>[2x]MTSRDGYQWTPETGLTQGVPSLGVISPPTNIEDTDKDGPWDVIVIGGGYCGLTATRDLTVAGFKTLLLEARDRIGGRSWSSNIDGYPYEMGGTWVHWHQSHVWREITRYKMHNALSPSFNFSRGVNHFQLRTNPTTSTYMTHEAEDELLRSALHKFTNVDGTNGRTVLPFPHDMFYVPEFRKYDEMSYSERIDQIRDELSLNERSSLEAFILLCSGGTLENSSFGEFLH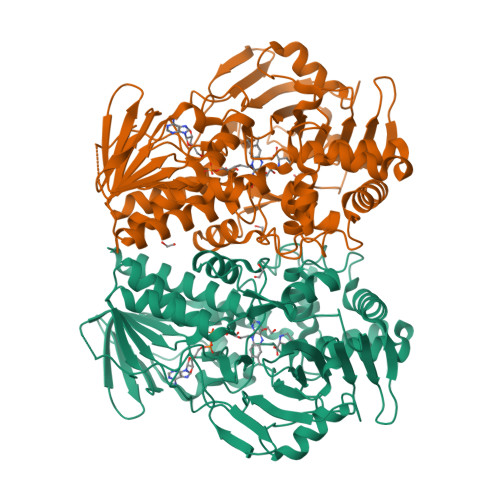WWAMSGYTYQGCMDCLMSYKFKDGQSAFARRFWEEAAGTGRLGYVFGCPVRSVVNERDAARVTARDGREFVAKRVVCTIPLNVLSTIQFSPALSTERISAMQAGHVSMCTKVHAEVDNKDMRSWTGIAYPFNKLCYAIGDGTTPAGNTHLVCFGNSANHIQPDEDVRETLKAVGQLAPGTFGVKRLVFHNWVKDEFAKGAWFFSRPGMVSECLQGLREKHGGVVFANSDWALGWRSFIDGAIEEGTRAARVVLEELGTKREVKARL>MIVRGINMTKIKLESPGFMVHKKLKSMSQSYGVMMTGVPAEVLGQMQAERSIPSINKTGNLKQQIAKEVSKVCHMMTEPTQSCGQASNDVCELLLGKIEAEKFHFTKYEALSADGDNLKNVLENTAPSSTNLLIRFEIDREDPPIVLVKTKNENFNPETAVKNKIYLLENKLYFIDKMGNLFNLGPGKKKCTQLFNAIGDSAEYSLCDPFVLEEPEKPEDFAISEIVDIFNEQKERFDFWIGSHSFTIYIPQTLGESPRQFYPYQAYFGSHTLQDWFVSDKDEYLSRIGIDKYIEKLAVLGKTTNTKERSDI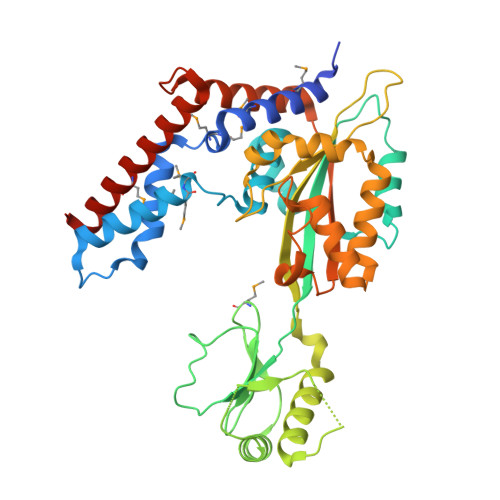YAEFFSKRGREAFFCAHLNEKRQPLRVKFKITEINPELALKNLQETQEFIDTHPGENPSDKVENYRNRAKLAMTEHLESLLDIKPESS[2x]> MRDAVTTLIKNYDLTGRYLDRNAMDELKAYFESGSARIAAAAMINANSA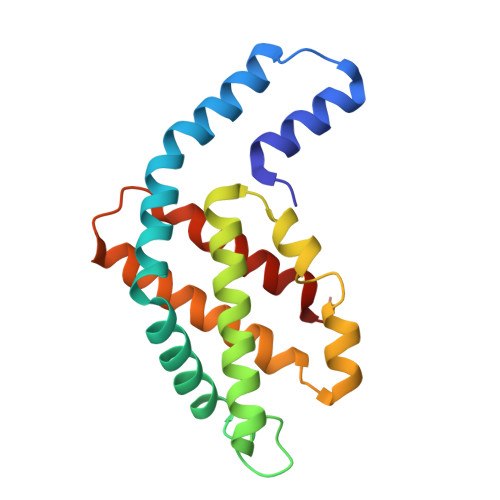TIVKRAAAQLFEEIPELIRPSGNAYTTRRFSACLRDMDYYLRYASYALIAADNNVLDERVLQGLRETYNSLGVPIGPTVRGIQIMKEMIEAMAEDSSLNSTDFIASPFDHMTRELSELSV> MALGDLLKMVNWTRNWFGFSCLFVLTLAVMLGLKLFLPSPVVAQSSSDFIQQGNQISIDGKSYPVAWGQWQEGGQTRTGLGDTGAMQFLGLDLLDNTSPNQQPVQWFSGDRQTLNARFVAPNRYLDVTSLLQGFGPLQAQGNTLVMPNTNAQILTVRDGRQSWGERVVLELSQPAFWQVSQAREEAVVTINASSTIGSQGNANAPGLQAIDQDDLGGKTSGGQQIRYRLERSGASSKVHFQLPVGYKLQVSTLTSPFRLVIDARADAPPVKTINWTEGITWQQRFVNISGGQFPVTTVTINPRSPGISLRPLMANPTMAQGTAPLVTIARDQRAAVAINAGFFNRNNQLPLGAVWSQQNWRSG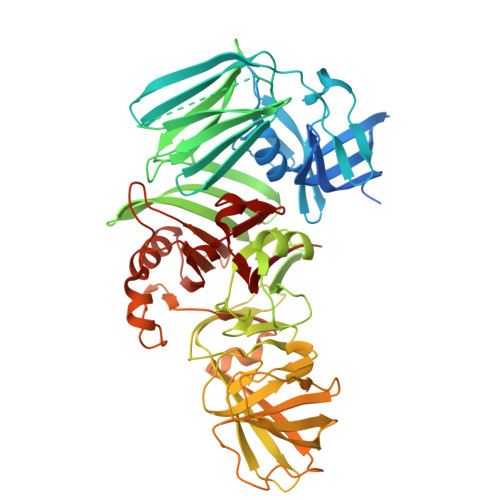PILNRGAIAWNDQGQTTFGRLSLSEIITTGSGQRLTANYLNSGYVQRGIARYTPAWGPSYIPLSDNEQVYVVQNSQVTAQYPLPKAGQQQMPIPSDGYLIIDRGNQIPAGVLAVGTTLNVNGRSTPEAFNAFPNGMGAGPLLIDQGRMVLNATGEGFSSAFQQQRASRSAIAVDRNGNIILVASHNRVGGAGASLGEFAQILQQLGAVNALNLDGGSSTSLALGGQLLDRSPVTAARVSNAIGVFVR4-(6-cyanopyridazin-3-yl)-N-[4-(propan-2-yl)phenyl]-3,4-dihydropyrazine-1(2H)-carboxamide 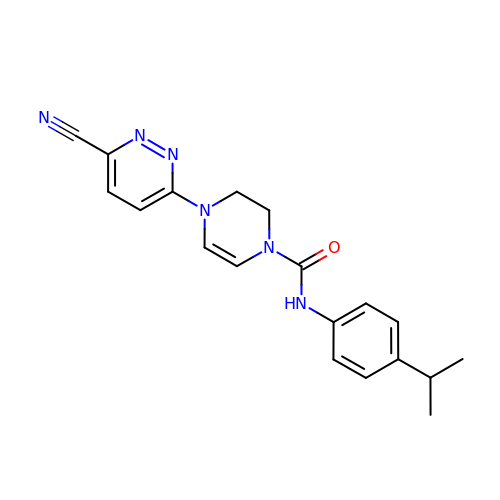| C19 H20 N6 O | UFOIVYYYFHTAEA-UHFFFAOYSA-N>[6x]MSEKKAVIGVVTISDRASKGIYEDISGKAIIDYLKDVIITPF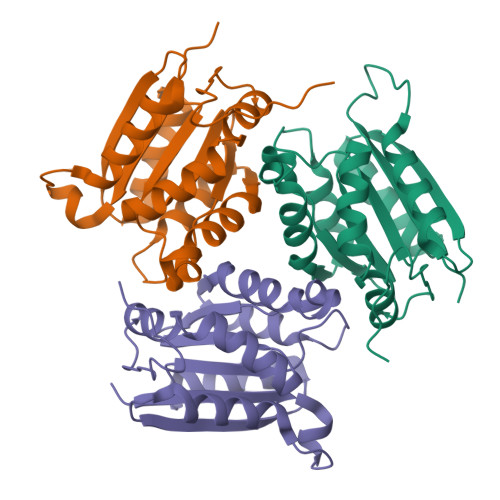EVEYRVIPDERDLIEKTLIELADEKGCSLILTTGGTGPAPRDVTPEATEAVCEKMLPGFGELMRQVSLKQVPTAILSRQTAGIRGSCLIVNLPGKPQSIKVCLDAVMPAIPYCIDLIGGAYIDTDPNKVKAFRPKK>[2x]SGISLDNSYKMDYPEMGLCIIINNKNFHKSTGMTSRSGTDVDAANLRETFRNLKYEVRNKNDLTREEIVELMRDVSKEDHSKRSSFVCVLLSHGE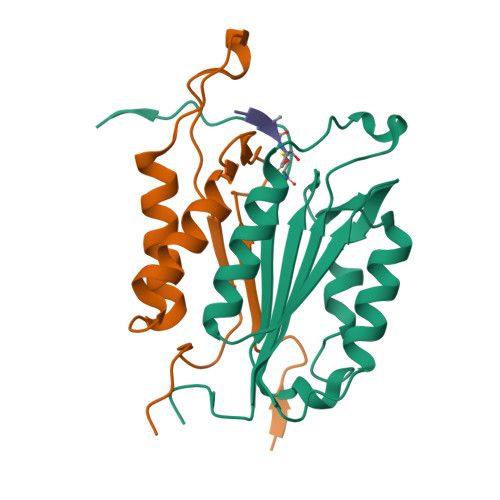EGIIFGTNGPVDLKKITNFFRGDRCRSLTGKPKLFIIQACRGTEDDCGIETD;>[2x]SGVDDDMACHKIPVEADFLYAYSTAPGYYSWRNSKDGSWFIQSLCAMLKQYADKLEFMHILTRVNRKVATEFESFSFDATFHAKKQIPCIVSMLTKELYFYHHHHHHH> MTSHFMLRRALLPLAIAALAGCSLAPTYERPQAPVASHWQAADAEGARAQALDWQTFIVDADLRRAVDTALSNNRSLRQALLDIEAARAQYRIQRADRLPSINANASGNRQRLPADLSQTGRSEVTSNYQVGLGLAEYEVDLFGRVRNLSEAALETYLATEEATRATQISLVAEVIQAYLTRDGALRRM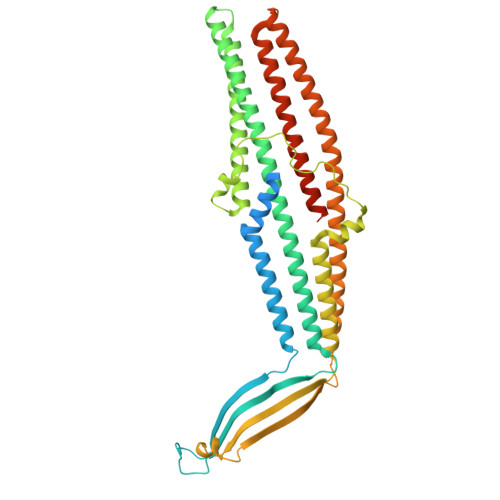ALVEQTLDSRMASLELVSQRRAAGAATALDYQEAVGLAEQARAERESTERQLRQADNALVLLLGTPDAARLLPATPRDDLMVLQDIAPGTSSELIERRPDILASEHRLKARNADIGAARAAFFPRISLTGSVGSSSAELSGLFDGGSRAWSFAPTLSLPIFAGGRNRANLDLAEVRQDAAVADYEGTIQTAFREVADALAATDTLRREEAARQALAGSSEAAMALAKARYEGGVDDYLRYLDAQRSTFSNQTTLIQISTERQIALVDLFRSLGGGWGQTEPMAGIGAEHHHHHH>[4x]ADTIVAVELDSYPNTDIGDPNYPHIGIDIKSVRSKSTARWNMQTGKVGTVHISYNSVSKRLS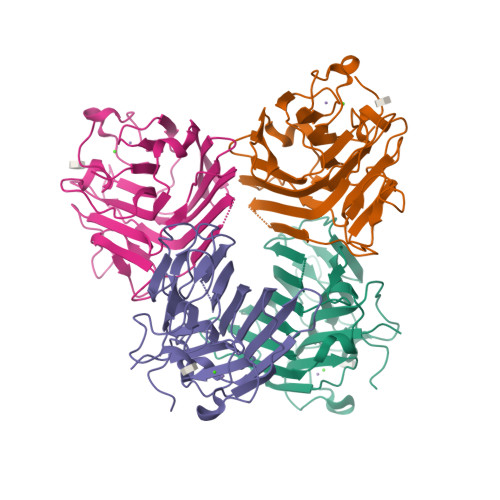AVVSYSGSSSTTVSYDVDLNNVLPEWVRVGLSATTGLYKQTNTILSWSFTSKLKTNSIADENSLHFSFHKFSQNPKDLILQGDASTDSDGNLQLTKVSSSGDPQGNSVGRALFYAPVHIWEKSAVVASFDATFTFLIKSPDREPADGITFFIANTDTTIPSGSGGRLLGLFPDAN>[2x]HHHHHHGSGAVKLSVSYRNGTLFIMVMHIKDLVTEDGADPNPYVKTYLLPDTHK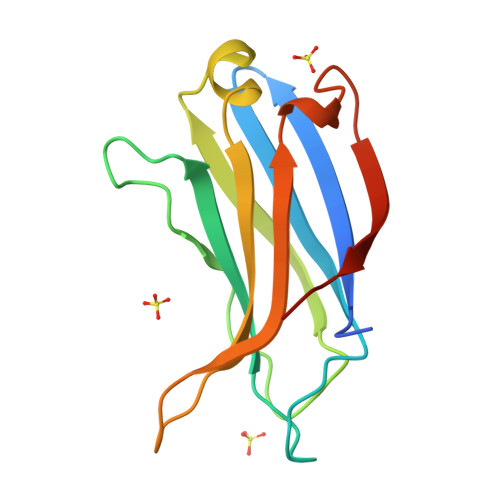TSKRKTKISRKTRNPTFNEMLVYSGYSKETLRQRELQLSVLSAESLRENFFLGGITLPLKDFNLSKETVKWYQLTAATYL>SNVPHKSSLPEGIAPGTVLRIRGLVPPNASRFHVNLLCGEEQGSDAALHFNPRLDTSEVVFNSKEQGSWGREERGPGVPFQRGQPFEVLIIASDDGFKAVVGDAQYHHFRHRLPLARVRLVEVGGDVQLDS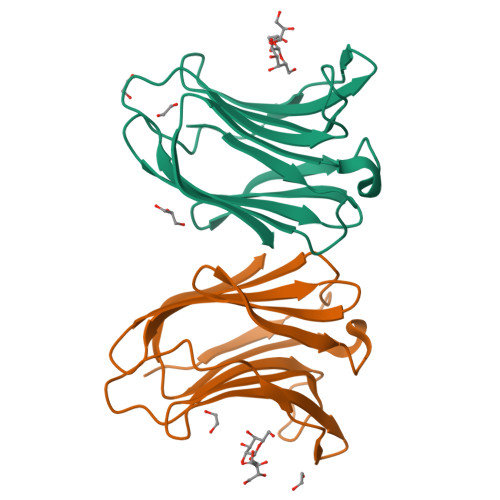VRIF[2x]>MQQGQMAGGRAITVFSPDGRLFQVEYAREAVKKGSTALGMKFANGVLLISDKKVRSRLIEQNSIEKIQLIDDYVAAVTSGLVADARVLVDFARISAQQEKVTYGSLVNIENLVKRVADQMQQYTQYGGVRPYGVSLIFAGIDQIGPRLFDCDPAGTINEYKATAIGSGKDAVVSFLEREYKENLPEKEAVTLGIKALKSSLEEGEELKAPEIASITVGNKYRIYDQEEVKKFL[7x];>[7x]MNQTLETGTTTVGITLKDAVIMATERRVTMENFIMHKNGKKLFQIDTYTGMTIAGLVGDAQVLVRYMKAELELYRLQRRVNMPIEAVATLLSNMLNQVKYMPYMVQLLVGGIDTAPHVFSIDAAGGSVEDIYASTGSGSPFVYGVLESQYSEKMTVDEGVDLVIRAISAAKQRDSASGGMIDVAVITRKDGYVQLPTDQIESRIRKLGLILHHHHHH;>[7x]MHHHHHHPPKRAALIQNLRDSYTETSSFAVIEEWAAGTLQEIEGIAKAAAEAHGVIRNSTYGRAQAEKSPEQLLGVLQRYQDLCHNVYCQAETIRTVIAIRIPEHKEEDNLGVAVQHAVLKIIDELEIKTLGSGEKSGSGGAPTPIGMYALREYLSARSTVEDKLLGSVDAESGKTKGGSQSPSLLL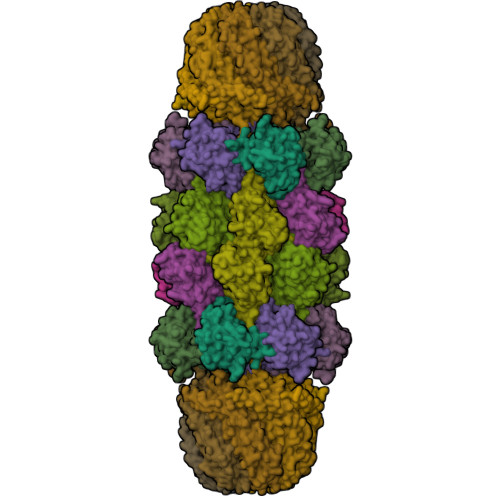ELRQIDADFMLKVELATTHLSTMVRAVINAYLLNWKKLIQPRTGSDHMVS>[2x]RKTYTLTDYLKNTYRLKLYSLRWISDHEYLYKQENNILVFNAEYGNSSVFLENSTFDEFGHSINDYSISPDGQFILLEYNYVKQWRHSYTASYDIYDLNKRQLITEERIPNNTQWVTWSPVGHKLAYVWNNDIYVKIEPNLPSYRITWTGKEDIIYNGITDWVYEEEVFSAYSALWWSPNGTFLAYAQFNDTEVPLIEYSFYSDESLQYPKTVRVPYPKAGAVNPTVKFFVVNTDSLSSVTNATSIQITAPASMLIGDHYLCDVTWATQERISLQWLRRIQNYSVMDICDYDESSGRWNCLVARQHIEMSTTGWVGRFRPSEPHFTLDGNSFYKIISNEEGYRHICYFQIDKK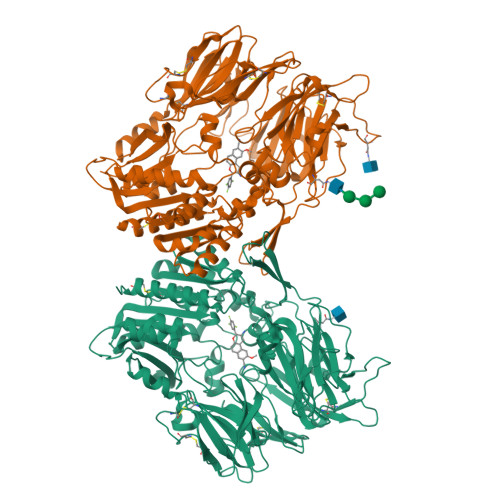DCTFITKGTWEVIGIEALTSDYLYYISNEYKGMPGGRNLYKIQLSDYTKVTCLSCELNPERCQYYSVSFSKEAKYYQLRCSGPGLPLYTLHSSVNDKGLRVLEDNSALDKMLQNVQMPSKKLDFIILNETKFWYQMILPPHFDKSKKYPLLLDVYAGPCSQKADTVFRLNWATYLASTENIIVASFDGRGSGYQGDKIMHAINRRLGTFEVEDQIEAARQFSKMGFVDNKRIAIWGWSYGGYVTSMVLGSGSGVFKCGIAVAPVSRWEYYDSVYTERYMGLPTPEDNLDHYRNSTVMSRAENFKQVEYLLIHGTADDNVHFQQSAQISKALVDVGVDFQAMWYTDEDHGIASSTAHQHIYTHMSHFIKQCFSLPGHHHHHH>[3x]SKPITPHYGPGHITPDWCGFGDARSDCGNKHTPKSLDIPQELCPKFSSRTGSSMFISMHWNNGSGFDAFDYSNCGVEKVFYEGVNFSPHRNYTCYQEGSSGWVSNKVGFYSKL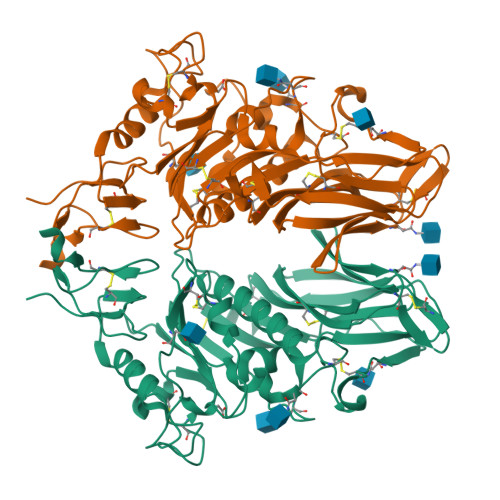YSMASTSRCIKLINLDPPTNFTNYRNGTCVGNGGTAKMPDNPQLVIFDAVTKLSTQFVLPNSSDGVSCTKHLVPFCYIDGGCFEMSGVCHPFGYYYESPSFYHGFYTNGTAGLHSYICDYLEMKPGVYNATTFGKFLIYPTKSYCMDTMNYTVPVQAVQSIWSENRQSDDAIGQACKSPYCIFYNKTKPYLAPNGADENHGDEEVRQMMQGLLVNSSCVSPQGSTPLALYSSEMIYIPNYGSCPQYYKLFETSSDENSDPLVPR>[2x]ELTPDQQTLLHFIMDSYNKQRMPQEITNKILKEEFSAEENFLILTEMATNHVQVLVEFTKKLPGFQTLDHEDQIALLKGSAVEAMFLRSAEIFNKK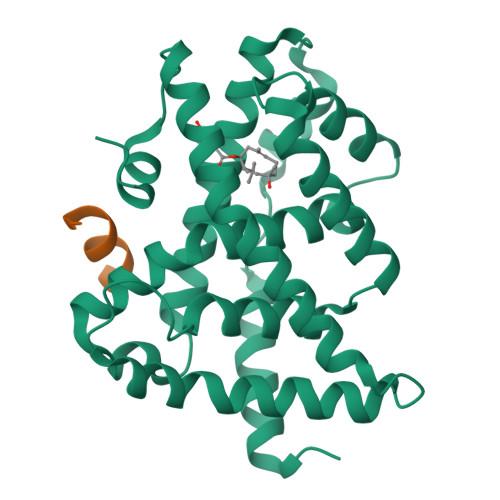LPSGHSDLLEERIRNSGISDEYITPMFSFYKSIGELKMTQEEYALLTAIVILSPDRQYIKDREAVEKLQEPLLDVLQKLCKIHQPENPQHFACLLGRLTELRTFNHHHAEMLMSWRVNDHKFTPLLCEIWDVQ;>[2x]NALLRYLLDKD> GSMEEFVKVRK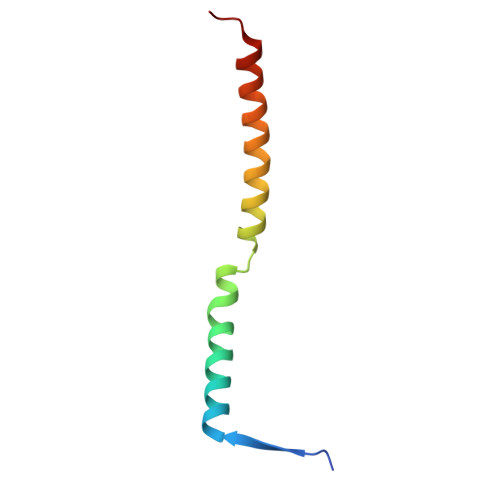KDLERLTTEVMQIRDFLPRILNGELLESFQKLKMVEKNLERKEQELEQLIMD[(2~{S})-2-azanyl-3-oxidanylidene-propyl] octanoate | C11 H21 N O3 | 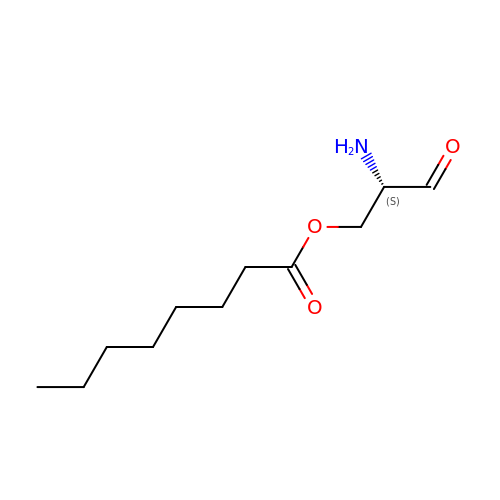CSUFCBOFZFUZNV-SNVBAGLBSA-N(2R)-2-(hexadecanoyloxy)propyl 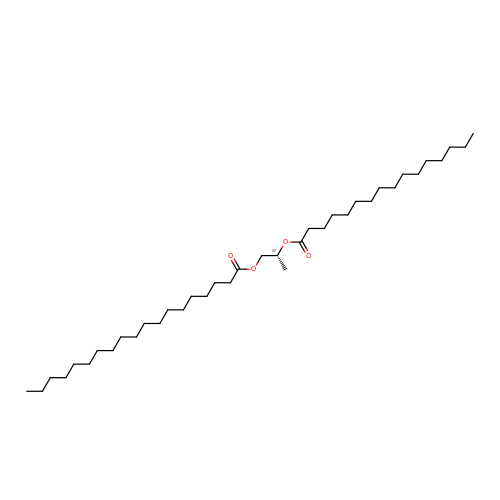nonadecanoate | C38 H74 O4 | AZEJVFRTMDKJQJ-PSXMRANNSA-N>AGSSSLEAVRRKIRSLQEQNYHLENEVARLKKLVGER[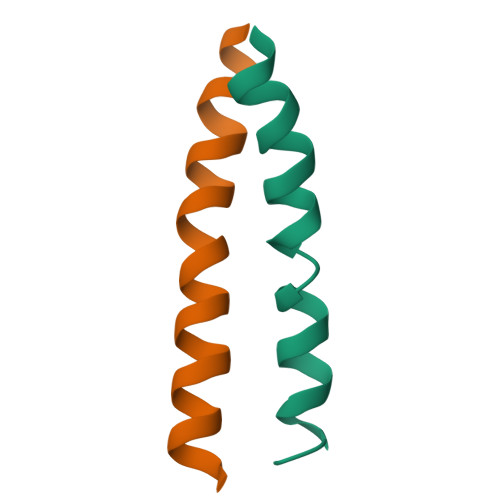2x]> MMIFFLSLSLESCSKEDDNNPSNSENNGGNNNLGTELDYDTFCFYYDWYGSEAIDGQYRHWAHAIAPDPNGGSGQNPGTIPGTQESIASNFYPQLGRYSSSDPNILTKHMDMFVMARTGVLALTWWNEQDETEAKRIGL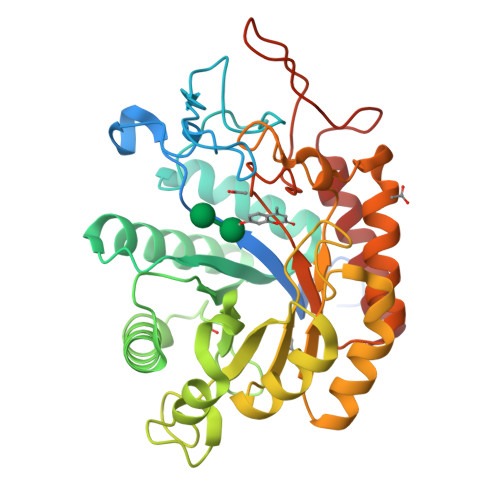ILDAADKKKIKVCFHLEPYPSRNVQNLRENIVKLITRYGNHPAFYRKDGKPLFFIYDSYLIEPSEWEKLLSPGGSITIRNTAYDALMIGLWTSSPTVQRPFILNAHFDGFYTYFAATGFTYGSTPTNWVSMQKWAKENGKIFIPSVGPGYIDTRIRPWNGSVIRTRTDGQYYDAMYRKAIEAGVSAISITSFNQWHEGSQIEPAVPYTSSEFTYLDYENREPDYYLTRTAYWVGKFRESKQ>TEARVWNARSLAEALSGTELFSSGEAQIELIEGAEASLYVIMREYGDLPVFVAPQGEQIIVEALLWPESDVTDATAFNEEVLLSRQLFPLSSIGLLNLPGEER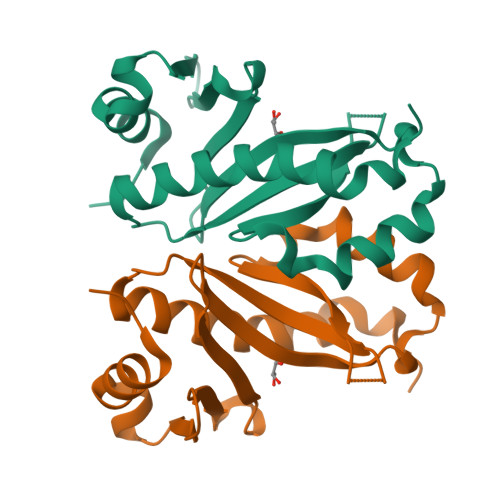CYSMFGALSTTSSLASVLHEIETLAGNVIRATEVYAGYLKARA[2x]>SEKLGDICFSLAYVPTAGKLTVVILAAKNLKKMDVGGLSDPYVKIHLMQNGKRLKKKKTTIKKNTLNPWYNESFSFEVP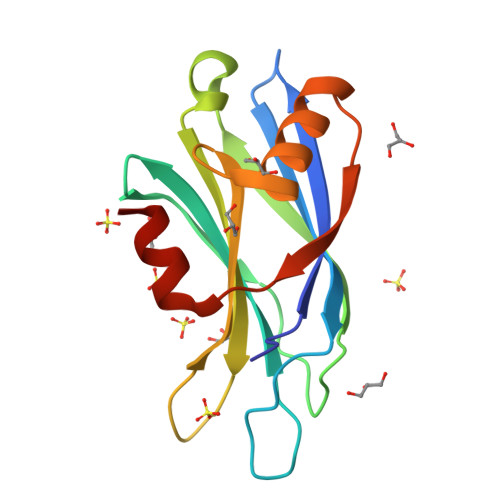FEQIQKVQVVVTVLDYDKIGKNDAIGKVFVGYNSTGAELRHWSDMLANPAAPIAQWHTLQVEEEVDAMLAVKK[4x]> MGSHHHHHHSQDPMAYSTREILLALCIRDSRVHGNGTL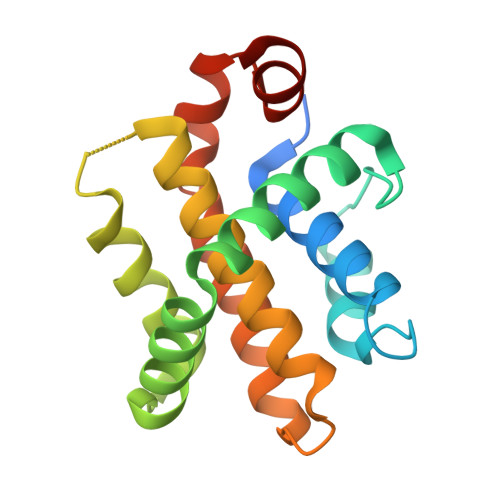HPVLELAARETPLRLSPEDTVVLRYHVLLEEIIERNSETFTETWNRFITHTEHVDLDFNSVFLEIFHRGDPSLGRALAWMAWCMHACRTLCCNQSTPYYVVDLSVRGMLEASEGLDGWIHQQGGWSTLIEDNIPG[(3~{S},8~{S},9~{S},10~{R},13~{R},14~{S},17~{R})-10,13-dimethyl-17-[(2~{R})-5-[[4-(2-morpholin-4-ylethoxy)phenyl]methylamino]-5-oxidanylidene-pentan-2-yl]-2,3,4,7,8,9,11,12,14,15,16,17-dodecahydro-1~{H}-cyclopenta[a]phenanthren-3-yl] 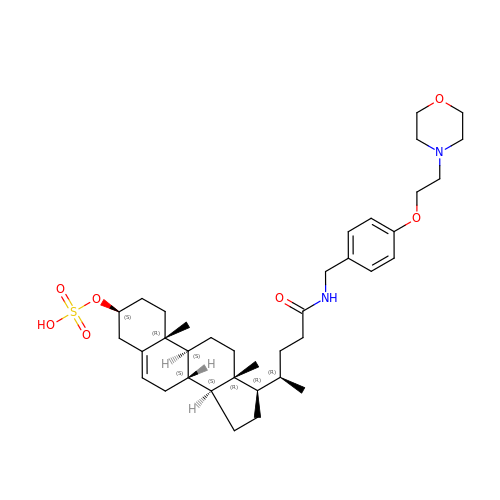hydrogen sulfate | C37 H56 N2 O7 S | YYAVRELUMNJNKQ-RMCWQMHZSA-N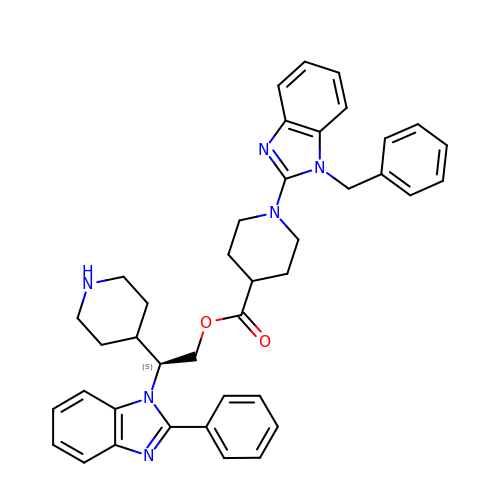(2S)-2-(2-phenyl-1H-benzimidazol-1-yl)-2-(piperidin-4-yl)ethyl 1-(1-benzyl-1H-benzimidazol-2-yl)piperidine-4-carboxylate | C40 H42 N6 O2 | WDALFJYWTFDSRP-DIPNUNPCSA-N> GSMVEATAQETDRPRFSFSIAAREGKARTGTIEMKRGVIRTPAFMPVGTAATVKALKPETVRATGADIILGNTYHLMLRPGAERIAKLCGLHSFMGWDRPIL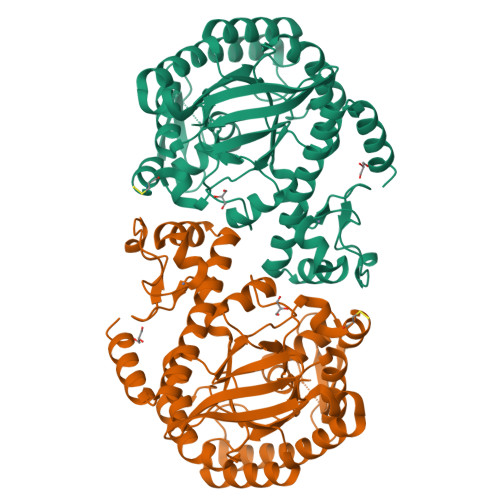TDSGGYQVMSLSSLTKQSEEGVTFKSHLDGSRHMLSPERSIEIQHLLGSDIVMAFDESTPYPATPSRAASSMERSMRWAKRSRDAFDSRKEQAENAALFGIQQGSVFENLRQQSADALAEIGFDGYAVGGLAVGEGQDEMFRVLDFSVPMLPDDKPHYLMGVGKPDDIVGAVERGIDMFDSVLPTRSGRNGQAFTWDGPINIRNARFSEDLKPLDSECHCAVCQKWSRAYIHHLIRAGEILGAMLMTEHNIAFYQQLMQKIRDSISEGRFSQFAQDFRARYFARNS3-(6-AMINO-PURIN-9-YL)-5-HYDROXYMETHYL-CYCLOPENTANE-1,2-DIOL | C11 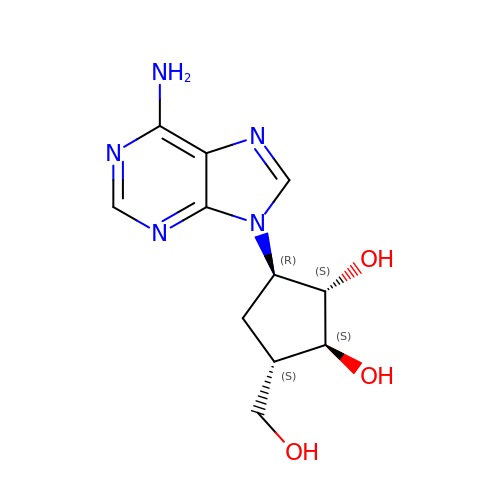H15 N5 O3 | UGRNVLGKAGREKS-FAYXRDSDSA-N> MAGASVKVAVRVRPFNSREMSRDSKCIIQMSGSTTTIVNPKQPKETPKSFSFDYSYWSHTSPEDINYASQKQVYRDIGEEMLQHAFEGYNVCIFAYGQTGAGKSYTMMGKQEKDQQGIIPQLCEDLFSRINDTTNDNMSYSVEVSYMEIYCERVRDLLNPKNKGNLRVREHPLL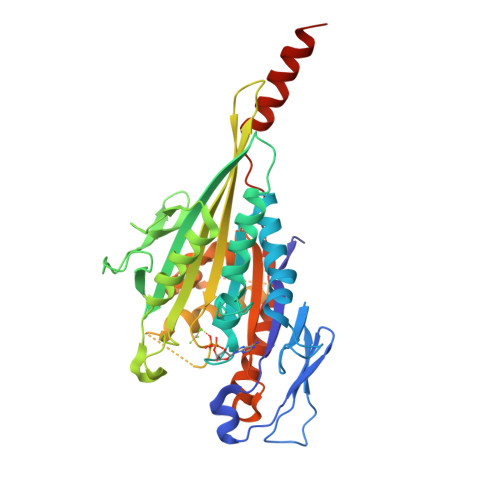GPYVEDLSKLAVTSYNDIQDLMDSGNKPRTVAATNMNETSSRSHAVFNIIFTQKRHDAETNITTEKVSKISLVDLAGSERADSTGAKGTRLKEGANINKSLTTLGKVISALAEMDSGPNKNKKKKKTDFIPYRDSVLTWLLRENLGGNSRTAMVAALSPADINYDETLSTLRYADRAKQIRCNAIINEDPNNKLIRELKDEVTRLRDLHHHHHHH> MGQQESTLGGAAGEPRSRGHAAGTSGGPGDHLHATPGMFVQHSTAIFSDRYKGQRVLGKGSFGEVILCKDKITGQECAVKVISKRQVKQKTDKESLLREVQLLKQLDHPNIMKLYEFFEDKGYFYLVGEVYTGGELFDEIISRKRFSEVDAARIIRQVLSGITYMHKNKIVHRDLKPENLLLESKSKDANIRIIDFGLSTHFEASKKMKDKIGTAYYIAPEVLHGTYDEKCDVWSTGVILYILLSGCPPFNGANEYDILKKVEKGKYTFELPQWKKVSESAKDLIRKMLTYVPSMRISARDALDHEWIQTYTKEQISVDVPSLDNAILNIRQFQGTQKLAQAALLYMGSKLTSQDETKELTAIFHKMDKNGDGQ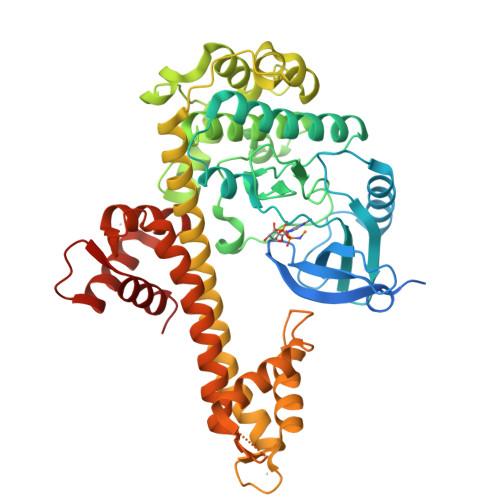LDRAELIEGYKELMRMKGQDASMLDASAVEHEVDQVLDAVDFDKNGYIEYSEFVTVAMDRKTLLSRERLERAFRMFDSDNSGKISSTELATIFGVSDVDSETWKSVLSEVDKNNDGEVDFDEFQQMLLKLCGN> QAMFERFTDRARRVIVLAQEEARMLNHNYIGTEHILLGLIHEGEGVAAKALESMGISLDAVRQEVEEIIGQGSQPTTGHIPFTPRAKKVLELSLREGLQMGHKYIGTE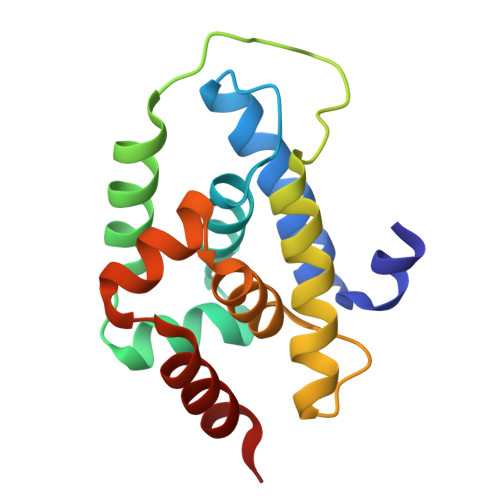FLLLGLIREGEGVAAQVLVKLGADLPRVRQQVIQLLSG>[4x]MSQSPAFGPRRGSSPRGAAGAAARRNESQDYLLMDSELGEDGCPQAPLPCYGYYPCFRGSDNRLAHRRQTVLREKGRRLANRGPAYMFSDRSTSLSIEEERFLDAAEYGNIPVVRKMLEECHSLNVNCVDYMGQNALQLAVANEHLEITELLLKKENLSRVGDALLLAISKGYVRIVEAILSHPAFAEGKRLATSPSQSELQQDDFYAYDEDGTRFSHDVTPIILAAHCQEYEIVHTLLRKGARIERPHD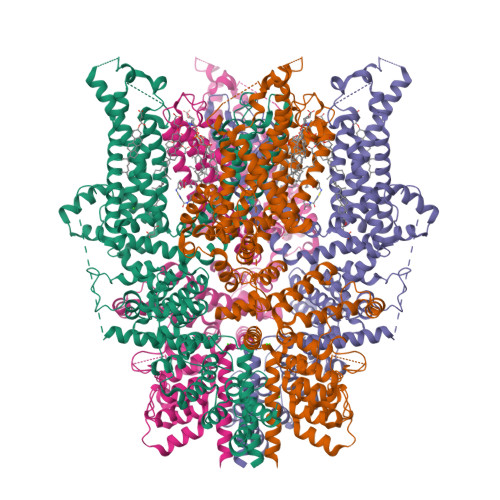YFCKCNDCNQKQKHDSFSHSRSRINAYKGLASPAYLSLSSEDPVMTALELSNELAVLANIEKEFKNDYKKLSMQCKDFVVGLLDLCRNTEEVEAILNGDVETLQSGDHGRPNLSRLKLAIKYEVKKFVAHPNCQQQLLSIWYENLSGLRQQTMAVKFLVVLAVAIGLPFLALIYWFAPCSKMGKIMRGPFMKFVAHAASFTIFLGLLVMNAADRFEGTKLLPNETSTDNAKQLFRMKTSCFSWMEMLIISWVIGMIWAECKEIWTQGPKEYLFELWNMLDFGMLAIFAASFIARFMAFWHASKAQSIIDANDTLKDLTKVTLGDNVKYYNLARIKWDPSDPQIISEGLYAIAVVLSFSRIAYILPANESFGPLQISLGRTVKDIFKFMVIFIMVFVAFMIGMFNLYSYYIGAKQNEAFTTVEESFKTLFWAIFGLSEVKSVVINYNHKFIENIGYVLYGVYNVTMVIVLLNMLIAMINSSFQEIEDDADVEWKFARAKLWFSYFEEGRTLPVPFNLVPSPKSLFYLLLKLKKWISELFQGHKKGFQEDAEMNKINEEKKLGILGSHEDLSKLSLDKKQVGHNKQPSIRSSEDFHLNSFNNPPRQYQKIMKRLIKRYVLQAQIDKESDEVNEGELKEIKQDISSLRYELLEEKSQNTEDLAELIRELGEKLSMEPNQEETNR>[4x]HHHHHHAIGYVWNTLYGWVDTGTGSLAAANLTARMQPISHHLAHPDTKRRFHELVCASGQIEHLTPIAAVAATDADILRAHSAAHLENMKRVSNLPTGGDTGDGITMMGNGGLEIARLSAGGAVELTRRVATGELSAGYALVNPPGHHAPHNAAMGFCIFNNTSVAAGYARAVLGMERVAILDWDVHHGNGTQDIWWNDPSVLTISLHQHLCFPPDSGYSTERGAGNGHGYNINVPLPPGSGNAAY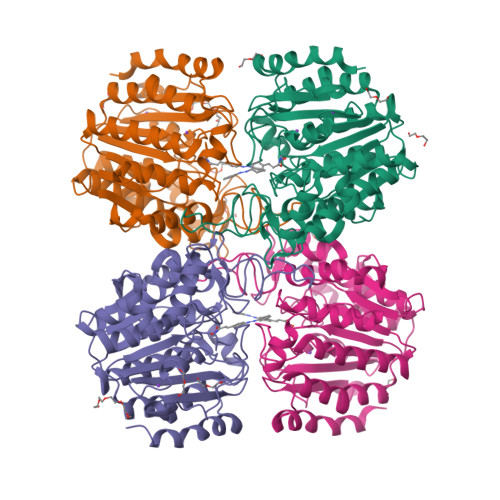LHAMDQVVLPALRAYRPQLIIVGSGFDASMLDPLARMMVTADGFRQMARRTIDCAADICDGRIVFVQEGGYSPHYLPFCGLAVIEELTGVRSLPDPYHEFLAGMGGNTLLDAERAAIEEIVPLLADIR> GSHMGEGEGVQLTAAQELMIQQLVAAQLQSNKRSFSDQPKVTPWPLGADPQSRDARQQRFAHFTELAIISVQEIVDFAKQVPGFLQLGREDQIALLKASTIEIMLLETARRYNHETESITFLKDFTYSKDDFHRAGLQVEFINPIFEFSRAMSSLGLDDAEYALLIAINIFSADRPNVQEPGRVEALQQPYVEALLSYTRIKRPQDQLRFPRMLMKLV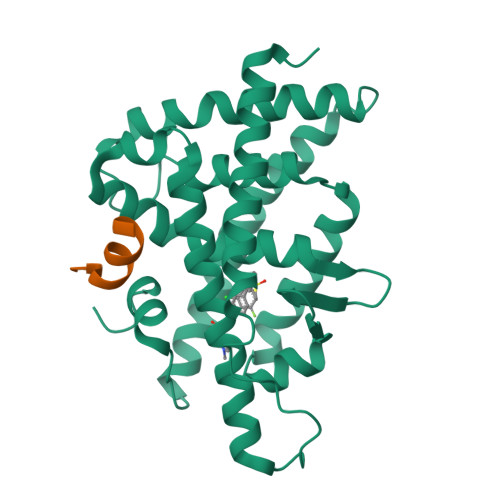SLRTLSSVHSEQVFALRLADAALPPLLSEIWDVHE;> KENALLRYLLDK beta-L-rhamnopyranose | C6 H12 O5 | 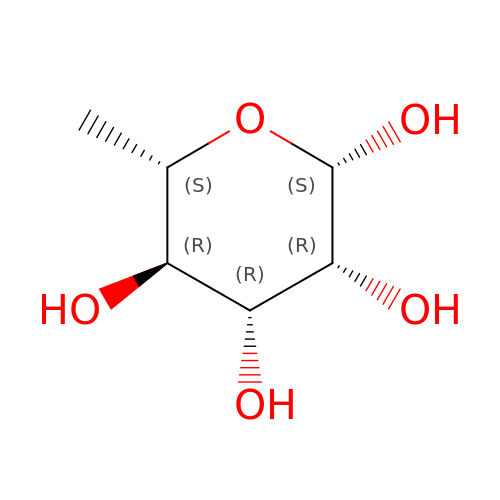SHZGCJCMOBCMKK-YJRYQGEOSA-N>MGSSHHHHHHSSGGNENLYFQGHMARASGSERHLLLIYTGGTLGMQSKGGVLVP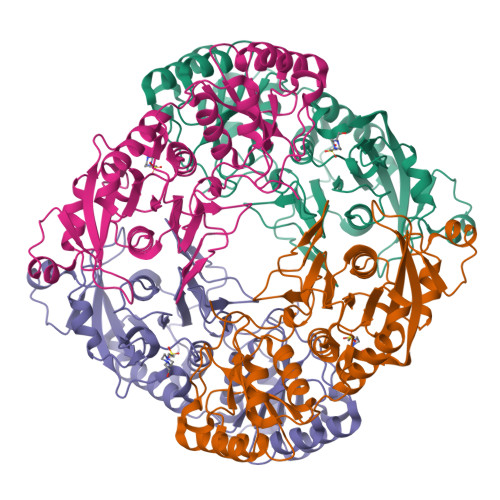GPGLVTLLRTLPMFHDKEFAQAQGLPDHALALPPASHGPRVLYTVLECQPLLDSSDMTIDDWIRIAKIIERHYEQYQGFVVIHGTDTMASGASMLSFMLENLHKPVILTGAQVPIRVLWNDARENLLGALLVAGQYIIPEVCLFMNSQLFRGNRVTKVDSQKFEAFCSPNLSPLATVGADVTIAWDLVRKVKWKDPLVVHSNMEHDVALLRLYPGIPASLVRAFLQPPLKGVVLETFGSGNGPSKPDLLQELRAAAQRGLIMVNCSQCLRGSVTPGYATSLAGANIVSGLDMTSEAALAKLSYVLGLPELSLERRQELLAKDLRGEMTLPT[8x]>MNRVLYPGTFDPITKGHGDLIERASRLFDHVIIAVAASPKKNPLFSLEQRVALAQEVTKHLPNVEVVGFS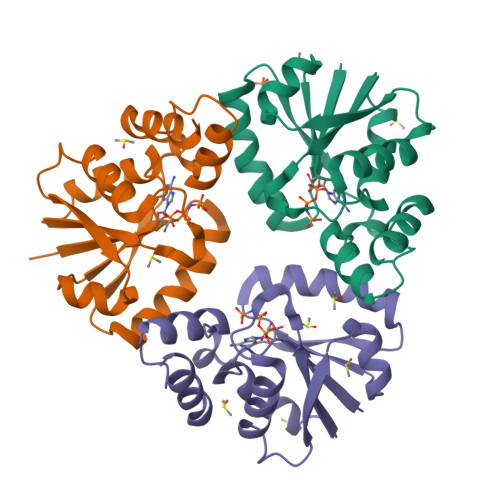TLLAHFVKEQKANVFLRGLRAVSDFEYEFQLANMNRQLAPDVESMFLTPSEKYSFISSTLVREIAALGGDISKFVHPAVADALAERFKR[6x]(5-{3-[5-(PIPERIDIN-1-YLMETHYL)-1H-INDOL-2-YL]-1H-INDAZOL-6-YL}-2H-1,2,3-TRIAZOL-4-YL)METHANOL 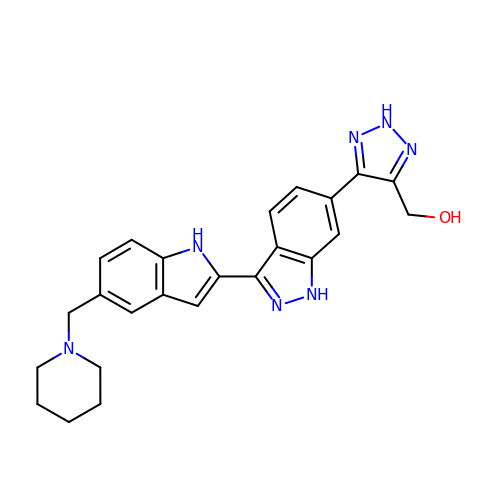| C24 H25 N7 O | FNWHPLLNMLOZTL-UHFFFAOYSA-N>[4x]GMNYQNDDLRIKEIKELLPPVALLEKFPATENAANTVAHARKAIHKILKGNDDRLLVVIGPCSIHDPVAAKEYATRLLALREELKD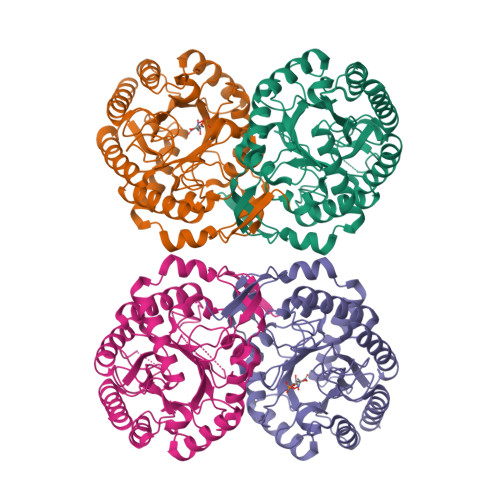ELEIVMRVYFEKPRTTVGWKGLINDPHMDNSFQINDGLRIARKLLLDINDSGLPAAGEFLDMITPQYLADLMSWGAIGARTTESQVHRELASGLSCPVGFKNGTDGTIKVAIDAINAAGAPHCFLSVTKWGHSAIVNTSGNGDCHIILRGGKEPNYSAKHVAEVKEGLNKAGLPAQVMIDFSHANSSKQFKKQMDVCADVCQQIAGGEKAIIGVMVESHLVEGNQSLESGEPLAYGKSITDACIGWEDTDALLRQLANAVKARRG N-[(S)-({[(benzyloxy)carbonyl]amino}methyl)(hydroxy)phosphoryl]-L-leucyl-L-leucine | C21 H34 N3 O7 P | 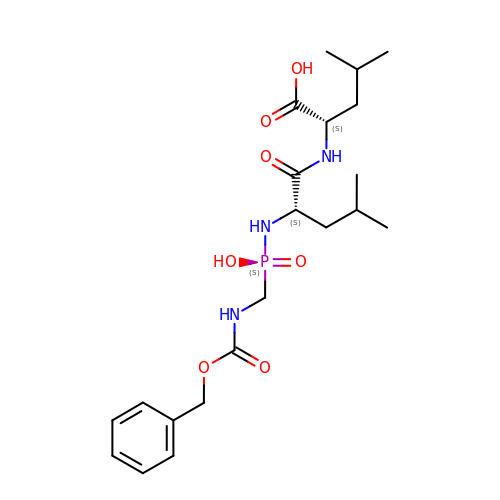ASUDVBNLLSQCDJ-ROUUACIJSA-N>MATKGTKRSYEQMETDGERQNATEIRASVGKMIDGIGRFYIQMCTELKLSDYEGRLIQNSLTIERMVLSAFDERRNKYLEEHPSAGKDPKKTGGPIYRRVDGKWRRELILYDKEEIRRIWRQANNGDDATAGLTHMMIWHSNLNDATYQRTRALVRTGMDPRMCSLMQGSTLPRRSGAAGAAVKGVGTMVMELIRMIKRGINDRNFWRGENGRRTRIAYERMCNILKGKFQTAAQRTMVDQVRESRNPGNAEFEDLIFLARSALILRGSVAHKSCLPACVYGSAV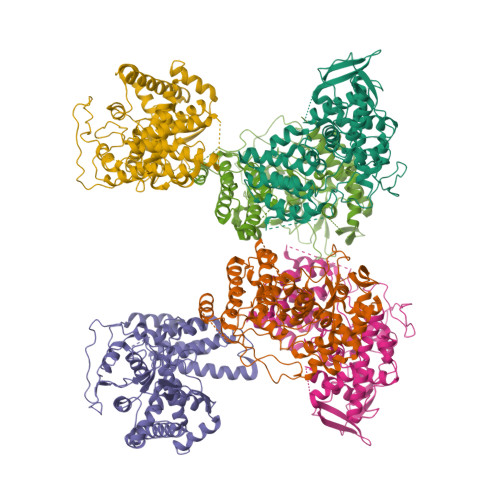ASGYDFEREGYSLVGIDPFRLLQNSQVYSLIRPNENPAHKSQLVWMACHSAAFEDLRVSSFIRGTKVVPRGKLSTRGVQIASNENMETMESSTLELRSRYWAIRTRSGGNTNQQRASSGQISIQPTFSVQRNLPFDRPTIMAAFTGNTEGRTSDMRTEIIRLMESARPEDVSFQGRGVFELSDEKATSPIVPSFDMSNEGSYFFGDNAEEYDN[6x]5-(4-fluorophenyl)-2-methyl-3~{H}-thieno[2,3-d]pyrimidin-4-one | C13 H9 F N2 O S | 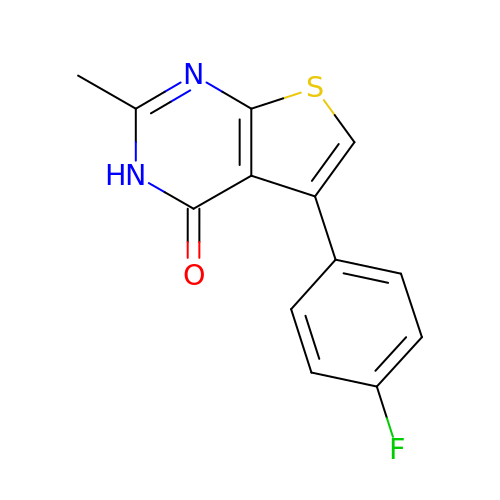PEYKEBUFADUZJK-UHFFFAOYSA-N>GSGIIEFHVIGNSLTPKANRRVLLWLVGLQNVFSHQLPRMPKEYIARLVFDPKHKTLALIKDGRVIGGICFRMFPTQGFTEIVFCAVTSNEQVKGYGTHLMNHLKEYHIKHNILYFLTYADEYAIGYFKKQGFSKDIKVPKSR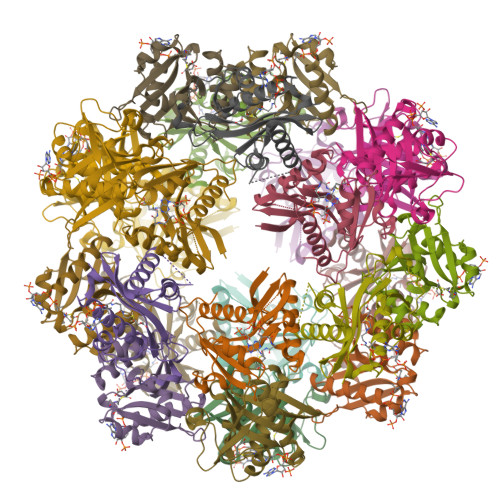YLGYIKDYEGATLMECELNPRIPYT[8x]>[2x]MENLIDFSGRDGLDRWLRATFPDVILSVGLTNYGSLMTSVPDLSHFEQMARQAKSEQEKDAVYSKALTEATRKAAPIAACALTSSKEMVKKGLQWFEDQIISEDGNFLVWHQNYEQLKKAPPSFEQLMGYQMSALNWRQSVGYGQLEETAVLVSQVIAQFSVPGTLVVTVQEMIKDMIARRGGGPKRGVS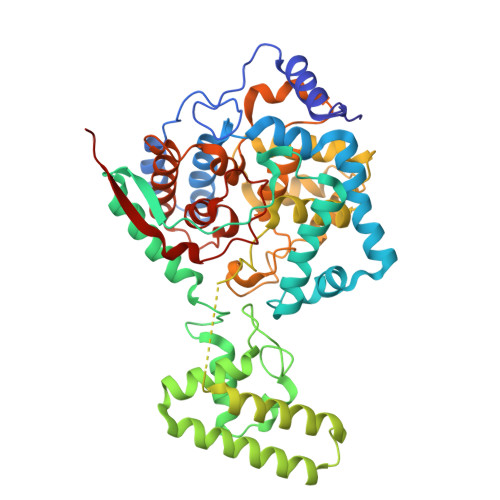EEHVRCCVDIMNGNLSALINPAWGDIDKKNKNGLMLLTTGIAKLRELYGPAAMVKVQQAADKFGEWGKAQDVLDQSRVQEIHQVLLKSIAESTSLGGGAAVFKNQIAQIDSVFSSYYWMWRAGITPESFPLLSDFLFELGQNARGSAKIIKTLDRIGLKWSKPLVNLFADSTFKMGRIHMHPAILTTGRLNEMGLCFGIIPASHPESAVNGSGFAKNILNVRTDGMNPSAQLIVQLFDIQRQSRTLSDLDVVSSEHLFHQILVGKRTAYQNAFQVKGNATDTKIVGFDPPKI> MAQKTFTVTADSGI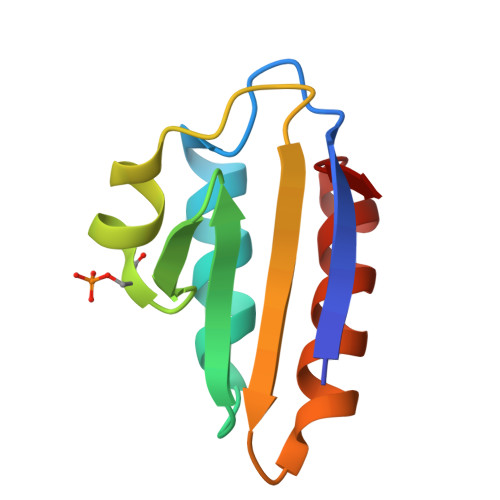HARPATTLVQAASKFDSDINLEFNGKTVNLKSIMGVMSLGIQKGATITISAEGSDEADALAALEDTMSKEGLGE>[4x]MGSDKIHHHHHHMKIDILDKGFVELVDVMGNDLSAVRAARVSFDMGLKDEERDRHLIEYLMKHGHETPFEHIVFTFHVKAPIFVARQWFRHRIASYNELSGRYSKLSY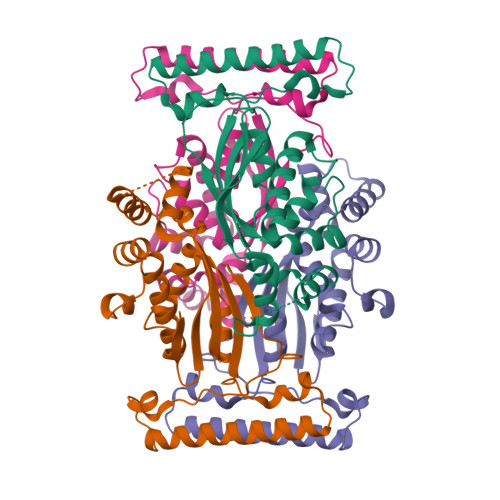EFYIPSPERLEGYKTTIPPERVTEKISEIVDKAYRTYLELIESGVPREVARIVLPLNLYTRFFWTVNARSLMNFLNLRADSHAQWEIQQYALAIARIFKEKCPWTFEAFLKYAYKGDILKEVQV> MSVYGLQRLYIAGAHADATSGKTFDTFDPATGELLARVQQASADDV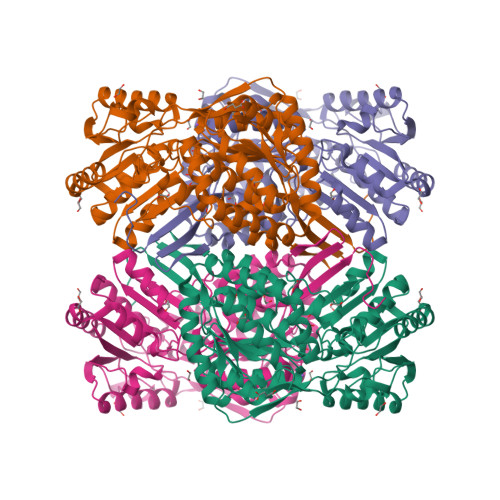DRAVASAREGQREWAAMTAMQRSRILRRAVELLRERNDALAELEMRDTGKPIAETRAVDIVTGADVIEYYAGLATAIEGLQVPLRPESFVYTRREPLGVCAGIGAWNYPIQIACWKSAPALAAGNAMIFKPSEVTPLSALKLAEIYTEAGVPAGVFNVVQGDGSVGALLSAHPGIAKVSFTGGVETGKKVMSLAGASSLKEVTMELGGKSPLIVFDDADLDRAADIAVTANFFSAGQVCTNGTRVFVQQAVKDAFVERVLARVARIRVGKPSDSDTNFGPLASAAQLDKVLGYIDSGKAEGAKLLAGGARLVNDHFASGQYVAPTVFGDCRDDMRIVREEIFGPVMSILSFETEDEAIARANATDYGLAAGVVTENLSRAHRAIHRLEAGICWINTWGESPAEMPVGGYKQSGVGRENGITTLEHYTRIKSVQVELGRYQPVFGHHHHHH> VPQDASTKKLSECLKRIGDELDSNME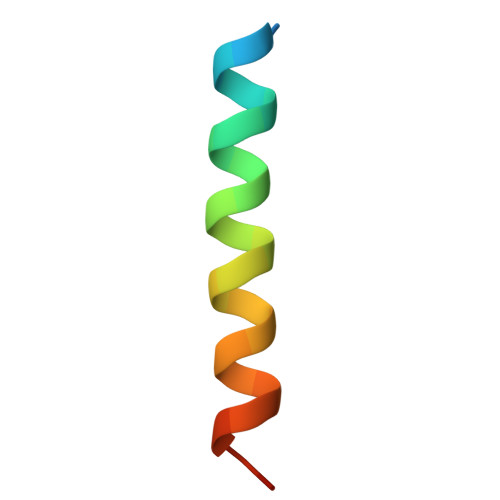LQ>MQDNSRYTHFLTQHYDAKPQGRDDRYCESIMRRRGLTSPCKDINTFIHGNKRSIKAICENKNGNPHRENLRISKSSFQVTTCKLHGGSPWPPCQYRATAGIRNVVVACENGLPVHLDQSIFRRP[2x]

Angiogenin (ANG), a 14-kDa basic protein is an angiogenic ribonuclease and member of the bovine pancreatic ribonuclease (RNase A) family (also known as RNase 5). Like RNase A, ANG cleaves preferentially on the 3′ side of pyrimidines and follows a transphosphorylation/hydrolysis mechanism. In addition, the crystal structure of human ANG has revealed that it has an RNase A fold and the catalytic triad (residues H13, K40 and H114) is conserved. The enzymatic activity of ANG is several orders of magnitude lower than that of RNase A towards conventional RNase substrates, but essential for its angiogenic effect.

In the native ANG structure F100 and V103 residues (located on β5 and β6 strands respectively) are in close proximity to the substrate binding site involving residue E108. The results from two variant structures F100I and V103I are analyzed here and both the variant residues are well defined in their respective electron density maps. The F100I variant implicated in ALS has retained only 39% of the enzymatic activity due to the significant loss of main chain interactions with S75 even though several of the side chain interactions have been retained with S75. The introduction of an Ile residue seems to have slightly increased flexibility in the vicinity of the mutated residue.>[2x]MRHPIPDYLASLVTELGAVNPGETAQYIPVLAEADPDRFGIALATPTGRLHCAGDADVEFTIQSASKPFTYAAALVDRGFAAVDRQVGLNPSGEAFNELSLEAESHRPDNAMINAGALAVHQLLVGPEASRKERLDRAVEIMSLLAGRRLSVDWETYESEMAVSDRNLSLAHMLRSYGVLQDSAEEIVAGYVAQCAVLVTVKDLAVMGACL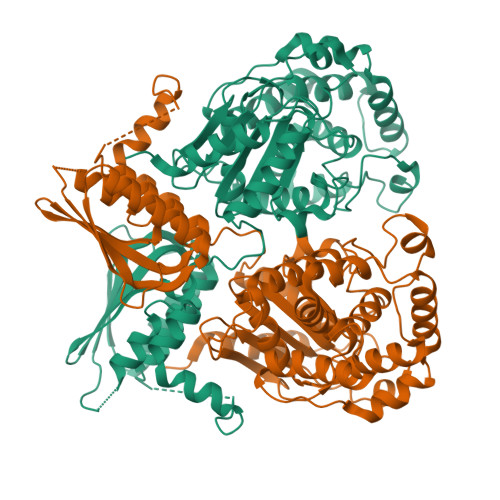ATGGIHPMTGERMLPSIVARRVVSVMTSSGMYDAAGQWLADVGIPAKSGVAGGVLGALPGRVGIGVFSPRLDEVGNSARGVLACRRLSEDFRLHLMDGDSLGGTAVRFVEREGDRVFLHLQGVIRFGGAEAVLDALTDLRTGAEKPGTGWDAAVYPRWQEAAADRAALSAATGGGAVHEAAAAAARDENDGPIRTVVLNLARVDRIDDVGRRLIAEGVRRLQADGVRVEVEDPERILPLEEAGAH> MSTATARRRVVLTGFGVISSIGTGVEEYTAGLRAGRSGARPITRFDTEGFGQNTACEVPDFEPGRWIHHVPLDDMGRAGQYAVAAARMAVDDAGLTEDDLGERQAVITVGTTDGESHDIAVLLE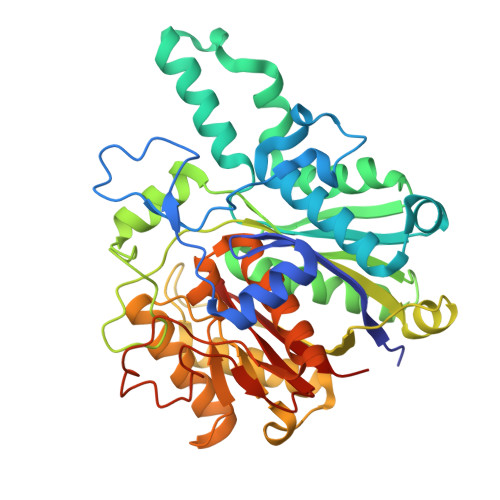QELAAGDPEAMDPVLARRINAGRLSTVIARELRMPNVEATTVTTACAAGNYSVGYGLDSIRSGEVDIALCGGADAVCRKAFALFKRFGALTPDVVRPFDKDRQGILTGEGAGILVLESLESALARGARIHAEVLGYGLSCDAAHPTAPNRDGIARGIRLALDDAGVEQEEIDFISAHGTGTKANDKTESAAIVDVYGDAPPRTVAVKSMLGHSMGAASALGAIACGLAIEHGFIPPTINHRETDPDCPLDVVPNRAVEADVRIVQNNSSAFAGNNAVLILGTYGE> ATSFAE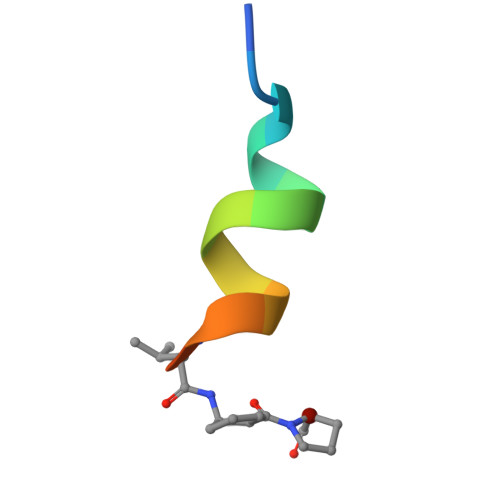YWALLXPA>[4x]EFMIIYRDLISHDEMFSDIYKIREIADGLCLEVEGKMVSRTEGNIDDSLIGGNASAEGPEGEGTESTVITGVDIVMNHHLQETSFTKEAYKKYIKDYMKSIKGKLEEQRPERVKPFMTGAA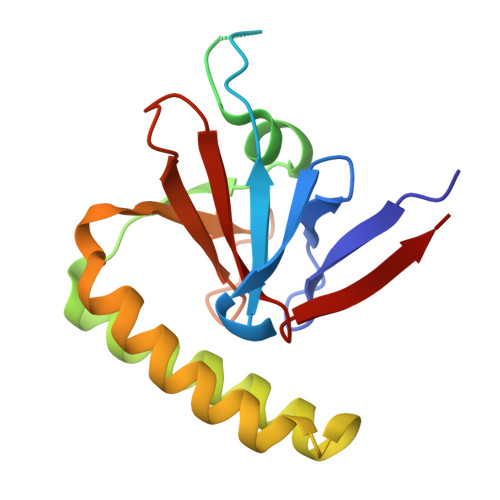EQIKHILANFKNYQFFIGENMNPDGMVALLDYREDGVTPYMIFFKDGLEMEKC FocA belongs to the widespread, evolutionarily ancient formate-nitrite transporter (FNT) family of pentameric anion channels and translocates formic acid bidirectionally. Central to the FNT family’s function are conserved histidine and threonine residues (H209 and T91 in E. coli FocA), both of which are essential for pH-dependent formate:H+ symport into fermenting E. coli cells. Here, we show the high-resolution structure of native E. coli FocA, together with the H209N variant, and describe the dynamic pore features that couple to the protonation state.

To identify if the FocA pentamer is inherently asymmetric and the observed flexibility at its cytoplasmic side is confined in the protomer, we further analyzed the cryo-EM data for native FocA without imposing any symmetry. The model reached a resolution of 2.87 Å (FSC = 0.143), with local resolution ranging from 2.7 to 3.1 Å. This calculation unambiguously confirms the 3D variability of the symmetric pentamer and shows that individual protomers have different degrees of resolvability for all regions identified to be of higher flexibility by the 3D variability analysis. The findings from the 3D variability analysis (A) were recapitulated within the asymmetric reconstruction, but regions with elevated flexibility exhibited asymmetric behavior. The N-terminal helix is clearly outlined at high resolution (1) but appears discontinuous in some regions (1′). Similar asymmetry is observed in region D98-L110 ((2) vs. (2′)) and the periplasmic region A227-L245 ((3) vs. (3′)). However, it will be important to investigate in future studies how this asymmetry is influenced by the membrane environment. Such asymmetry can have various implications, which may include: (a) protomers working independently of each other in formate/formic acid translocation, as hypothesized previously; (b) allosteric communication due to distinct thermal fluctuations of side chains that may reach several kcal mol‒1 of entropic contributions; (c) modulating protein-protein interactions via conformational selection mechanisms.

>[5x]MKADNPFDLLLPAAMAKVAEEAGVYKATKHPLKTFYLAITAGVFISIAFVFYITATTGTGTMPFGMAKLVGGICFSLGLILCVVCGADLFTSTVLIVVAKASGRITWGQLAKNWLNVYFGNLVGALLFVLLMWLSGEYMTANGQWGLNVLQTADHKVHHTFIEAVCLGILANLMVCLAVWMSYSGRSLMDKAFIMVLPVAMFVASGFEHSIANMFMIPMGIVIRDFASPEFWTAVGSAPENFSHLTVMNFITDNLIPVTIGNIIGGGLLVGLTYWVIYLRENDHH2-[(2~{R})-1-ethylimidazolidin-2-yl]-6-pyridin-2-yl-pyridine | C15 H18 N4 | 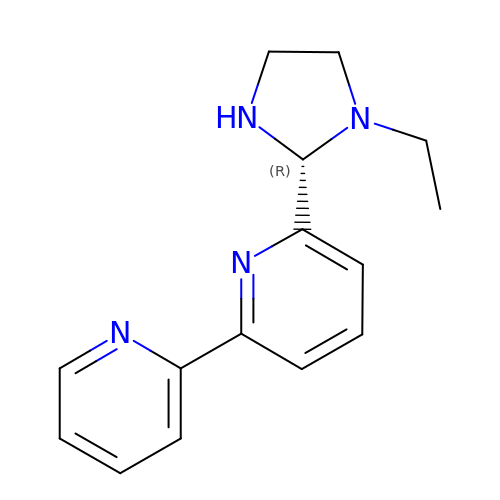KCAOHIFEVJIEQE-OAHLLOKOSA-N> MNPIHDRTSDYHKYLKVKQGDSDLFKLTVSDKRYIWYNPDPKERDSY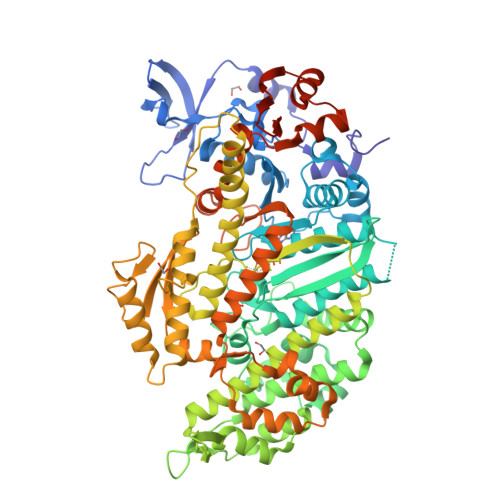ECGEIVSETSDSFTFKTVDGQDRQVKKDDANQRNPIKFDGVEDMSELSYLNEPAVFHNLRVRYNQDLIYTYSGLFLVAVNPFKRIPIYTQEMVDIFKGRRRNEVAPHIFAISDVAYRSMLDDRQNQSLLITGESGAGKTENTKKVIQYLASVAGRNQANGSGVLEQQILQANPILEAFGNAKTTRNNNSSRFGKFIEIQFNSAGFISGASIQSYLLEKSRVVFQSETERNYHIFYQLLAGATAEEKKALHLAGPESFNYLNQSGCVDIKGVSDSEEFKITRQAMDIVGFSQEEQMSIFKIIAGILHLGNIKFEKGAGEGAVLKDKTALNAASTVFGVNPSVLEKALMEPRILAGRDLVAQHLNVEKSSSSRDALVKALYGRLFLWLVKKINNVLCQERKAYFIGVLDIEGFEIFKVNSFEQLCINYTNEKLQQFFNHHMFKLEQEEYLKEKINWTFIDFGLDSQATIDLIDGRQPPGILALLDEQSVFPNATDNTLITKLHSHFSKKNAKYEEPRFSKTEFGVTHYAGQVMYEIQDWLEKNKDPLQQDLELCFKDSSDNVVTKLFNDPNIASRAKKGANFITVAAQYKEQLASLMATLETTNPHFVRCIIPNNKQLPAKLEDKVVLDQLRCNGVLEGIRITRKGFPNRIIYADFVKRYYLLAPNVPRDAEDSQKATDAVLKHLNIDPEQYRFGITKIFFRAGQLARIEEARELRGDYKDDDDK>[6x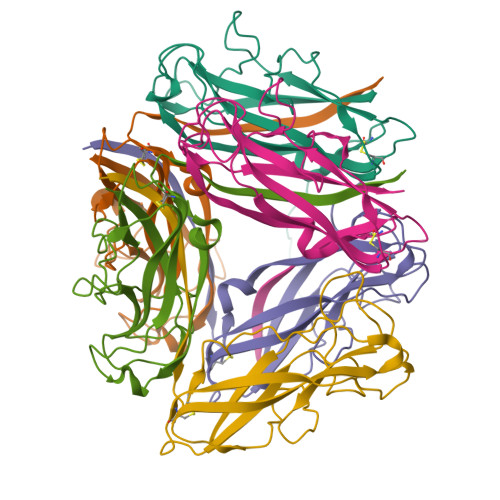]MKIKTLAIVVLSALSLSSTAALAAATTVNGGTVHFKGEVVNAACAVDAGSVDQTVQLGQVRTASLAQEGATSSAVGFNIQLNDCDTNVASKAAVAFLGTAIDAGHTNVLALQSSAAGSATNVGVQILDRTGAALTLDGATFSSETTLNNGTNTIPFQARYFATGAATPGAANADATFKVQYQ>EAKKEIPLKYGATNEGKRQDPAMQKFRDNRLGAFIHWGLYAIPGGEWNGKVYGGAAEWLKSWAKVPADEWLKLMDQWNPTKFDAKKWAKMAKEMGTKYVKITTKHHEGFCLWPSKYTKYTVANTPYKRDILGELVKAYNDEGIDVHFYFSVMDWSNPDYRYDIKSKEDSIAFSRFLEFTDNQLKELATRYPTVKDFWFDGTWDASVKKNGWWTAHAEQMLKELVPGVAINSRLRADDKGKRHFDSNGRLMGDYESGYQRRLPDPVKDLKVTQWDWEACMTIPENQWGYHKDWSLSYVKTPIEVIDRIVHAVSMGGNMVVNFGPQADGDFRPEEKAMATAIGKWMNRYGKA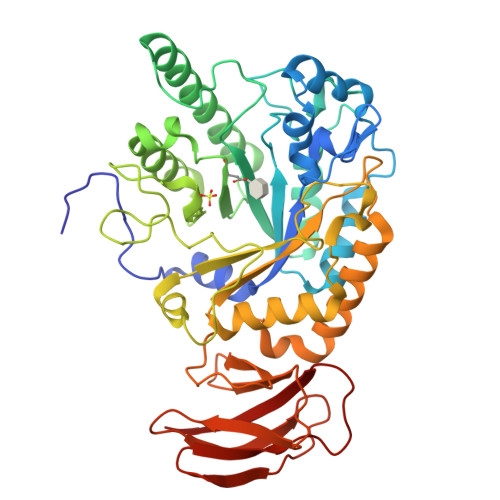VYACDYAGFEKQDWGYYTRGKNDEVYMVVFNQPYSERLIVKTPKGITVEKATLLTTGEDITVVETTRNEYNVSVPKKNPGEPYVIQLKVRAAK[4x]One enzyme in particular, 2-aminomuconate-6-semialdehyde dehydrogenase (AMSDH), is responsible for oxidizing the unstable metabolic intermediate 2-aminomuconate-6-semialdehyde (2-AMS) to 2-aminomuconate (2-AM). On the basis of sequence alignment, AMSDH is a member of the hydroxymuconic-semialdehyde dehydrogenase (HMSDH) family under the aldehyde dehydrogenase (ALDH) superfamily. The complete AMSDH model includes four polypeptides per asymmetric unit describing one homotetramer. Each monomer of AMSDH contains three domains: a subunit interaction domain, a catalytic domain and an NAD+ binding domain.

In the structure of the co-crystallized binary complex, an NAD+ molecule is present in an extended, anti-conformation in the amino-terminal, co-substrate-binding domain of each monomer. The electron density map of NAD+ is well defined, and the interactions between the protein and NAD+ are equivalent in all four subunits as shown in Fig. 2e. The NAD+-bound AMSDH structure is similar to the ligand-free structure with an aligned r.m.s.d. of 0.239 Å. Residues that belong to the NAD+-binding pocket are also well aligned with the exception of Cys302, Arg108 and Leu116. On binding NAD+, the thiol moiety of Cys302 rotates so that the sulfur is 2.3 Å closer to the substrate-binding pocket and away from the nicotinamide head of NAD+. Examining the wild-type AMSDH structures shows that in the NAD+-bound binary complex, Glu268 adopts a ‘passive’ conformation, pointing away from the substrate-binding pocket, and forms hydrogen bonds with both NE of Trp177 (3.2 Å distance) and the backbone oxygen of Phe470 (3.6 Å) to leave space for the reduction of NAD+. Its electron density is very well resolved and the side chain B-factor is close to average: 28.2 Å2/28.5 Å2. The thiol moiety of Cys302 is 7.14 Å from Glu268 and is unlikely to form interactions. The electron density for the side chain of Arg120 is partially missing in the binary complex structure but very well resolved in both ternary complex structures.

>[4x]MNTLPSQVWRTNIGSAPSQLLNYIDGNFVTSASSFANINPVNGKLISDVFEADAKQVNEAVVAAQNALKGPWGKLSVQDRAALIHKIADGIQARFEEFVAAEVADTGRPVHQARTLDIPRAIANFRTFADLAKTSHTDLFEMSTSDGSGALNYTVRKPLGVIGVISPWNLPLLLFTWKVAPALACGNTVVAKPSEESPSSATLLAEVMHDAGVPPGVFNLIHGFGKDSAGEFLTQHPGISALTFTGESKTGSTIMKAVADGVKEVSFELGGKNAAVVFADADLDAAIEGVLRSSFTNSGQVCLCSERVYVHRSIFDEFVSGLKVEAERLVVGYPDQDGVNMGPLISHGHRDKVLSYYRLAVDEGATVVTGGGVPKFNDERDQGAYVQPTIWTGLSDKARCVTEEIFGPVCHISPFDDEDEVINRVNDSNYGLACAIWTTNLSRAHRVSRQIHVGLVWVNTWYLRDLRTPFGGVKLSGLGREGGRFSMDFYSDIANICIKI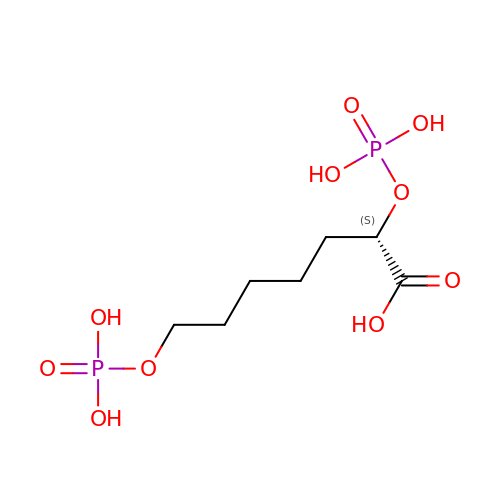(2S)-2,7-bis(phosphonooxy)heptanoic acid | C7 H16 O10 P2 | OZYHUBGACYJJJF-LURJTMIESA-N>SSFEGQMAEYPTISIDRFDRENLRARAYFLSHCHKDHMKGLRAPTLKRRLECSLKVYLYCSPVTKELLLTSPKYRFWKKRIISIEIETPTQISLVDEASGEKEEIVVTLLPAGHCPGSVMFLFQGNNGTVLYTGDFRLAQGEAARMELLHSGGRVKDIQSVYLDTTFCDPRFYQIPSREECLSGVLELVRSWITRSPYHVVWLNCKAAYGYEYLFTNLSEELGVQVHVNKLDMFRNMPEILHHLTTDRNTQIHACRHPKAEEYFQWSKLPCGITSRNRIPLHIISIKPSTMWFGERSRKTNVIVRTGESSYRACFSFHSSYSEIKDFLSYLCPVNAYPN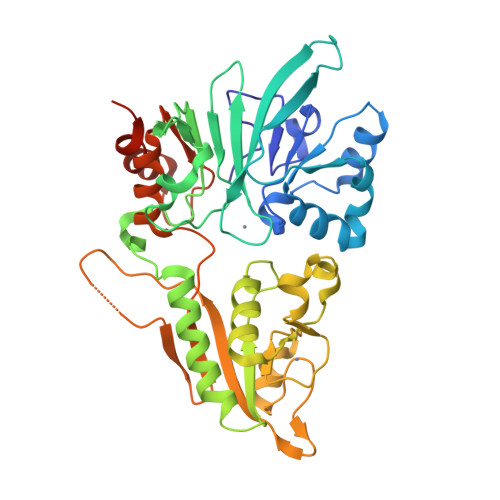VIPVGTTMDKVVEILKPLCRSSQSTEPKKGENLYFQ[2x]> MELKNSISDYTEAEFVQLLKEIEKENVAATDDVLDVLLEHFVKITEHPDGTDLIYYPSDNRDDSPEGIVKEIKEWRAANGKPGFKQG;> KRNKPGKATGKGKPVNNKWLNNAGKDLGSPVPDRIANKLRDKEFKSFDDFRKKFWEEVSKDPELSKQFSRNNNDRMKVGKAPKTRTQDVSGKRTSFELHHEKPISQNGGVYDMDNISVVTPKRHID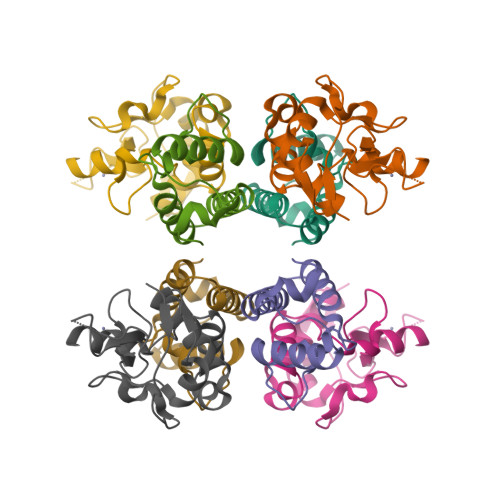IARGK> EAQKQYWVCNSSDASISYTYCDKMQYPISINVNPCIELKG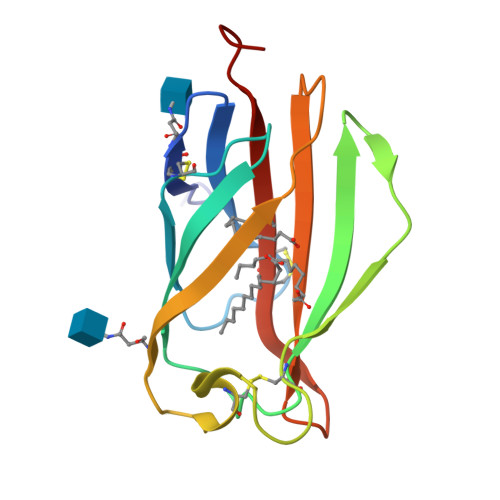SKGLLHIFYIPRRDLKQLYFNLYITVNTMNLPKRKEVICRGSDDDYSFCRALKGETVNTTISFSFKGIKFSKGKYKCVVEAISGSPEEMLFCLEFVILHQPNSN> GAEIPKEML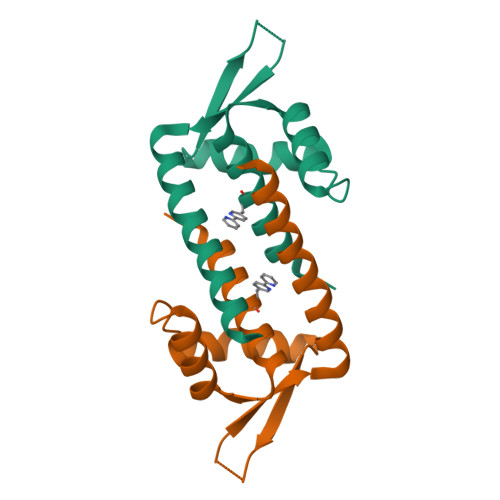RAQTNXILLNVLKQGDNYVYGIIKQVKEASNGEMELNEATLYTIFKRLEKDGIISSYWGDESQGGRRKYYRLTEIGHENMRLVSESWSRVDKIIENLEANKKSEAIKSRGGSGGWSHPQFEK>SMLELPPVASLKGKSITSAEQFSRADIYALIHLASAMQRKIDAGEVLNLLQGRIMTPLFFEDSSRTFSSFCAAMIRLGGSVVNFKVEASSINKGETLADTIRTLDSYSDVLVMRHPRQDAIEEAL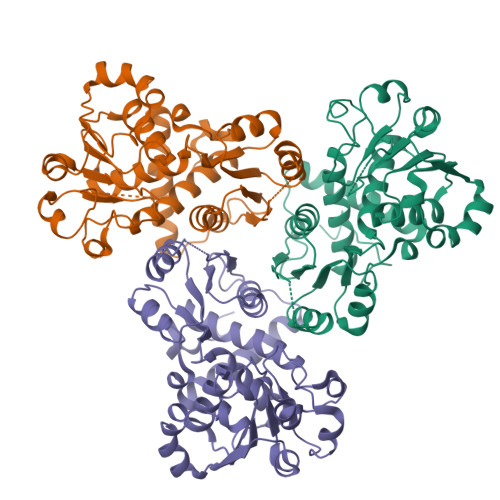SVAQHPILNAGNGAGEHPTQALLDTLTIHSELGSVDGITIALIGDLKMGRTVHSLLKLLVRNFSIKCVFLVAPDALQMPQDVLEPLQHEIATKGVIIHRTHALTDEVMQKSDVLYTTRLQKERFMASTSDDAAALQSFAAKADITIDAARMRLAKEKMIVMHPLPRNDELSTTVDADPRAAYFRQMRYGMFMRMAILWSVLA[6x]> MGQQPGKVLGDQRREPQGLSEAARWNSKENLLAGPSENDPNLFVAL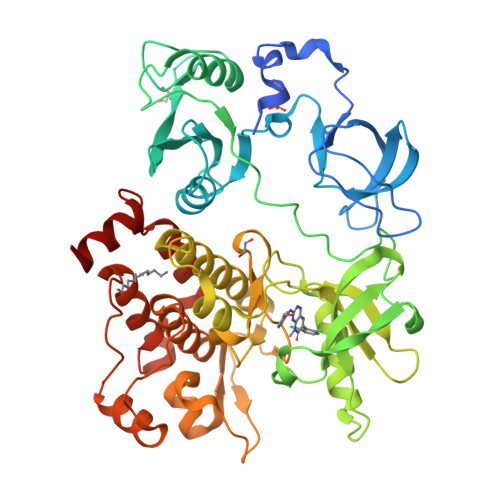YDFVASGDNTLSITKGEKLRVLGYNHNGEWCEAQTKNGQGWVPSNYITPVNSLEKHSWYHGPVSRNAAEYLLSSGINGSFLVRESESSPGQRSISLRYEGRVYHYRINTASDGKLYVSSESRFNTLAELVHHHSTVADGLITTLHYPAPKRNKPTVYGVSPNYDKWEMERTDITMKHKLGGGQYGEVYEGVWKKYSLTVAVKTLKEDTMEVEEFLKEAAVMKEIKHPNLVQLLGVCTREPPFYIITEFMTYGNLLDYLRECNRQEVNAVVLLYMATQISSAMEYLEKKNFIHRNLAARNCLVGENHLVKVADFGLSRLMTGDTYTAHAGAKFPIKWTAPESLAYNKFSIKSDVWAFGVLLWEIATYGMSPYPGIDLSQVYELLEKDYRMERPEGCPEKVYELMRACWQWNPSDRPSFAEIHQAFETMFQESSISDEVEKELGKENLYGQ>[2x]HHHHHHFNLPPGNYKKPKLLYCSNGGHFLRILPDGTVDGTRDRSDQHI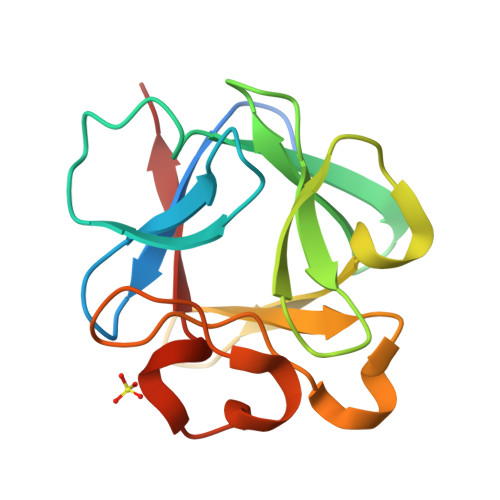QLQLSAESVGEVYIKSTETGQYLAMDTAGLLYGSQTPNEECLFLERLEENGYNTYISKKHAEKNWFVGLKKNGSCKRGPRTHYGQKAILFLPLPVSSD>[3x]MNQNLLVTKRDGSTERINLDKIHRVLDWAAEGLHNVSISQVELRSHIQFYDGIKTSDIHETIIKAAADLISRDAPDYQYLAARLAIFHLRKKAYGQFEPPALYDHVVKMVEMGKYDNHLLEDYTEEEFKQMDTFIDHDRDMTFSYAAVKQLEGKYLVQNRVTGEIYESAQFLYILVAACLFSNYPRET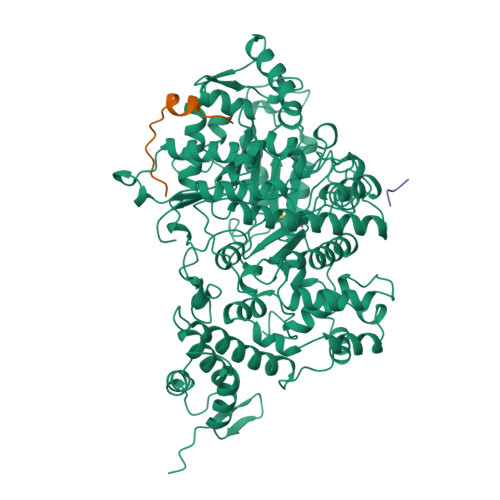RLQYVKRFYDAVSTFKISLPTPIMSGVRTPTRQFSSCVLIECGDSLDSINATSSAIVKYVSQRAGIGINAGRIRALGSPIRGGEAFHTGCIPFYKHFQTAVKSCSQGGVRGGAATLFYPMWHLEVESLLVLKNNRGVEGNRVRHMDYGVQINKLMYTRLLKGEDITLFSPSDVPGLYDAFFADQEEFERLYTKYEKDDSIRKQRVKAVELFSLMMQERASTGRIYIQNVDHCNTHSPFDPAIAPVRQSNLCLDIALPTKPLNDVNDENGEIALCTLSAFNLGAINNLDELEELAILAVRALDALLDYQDYPIPAAKRGAMGRRTLGIGVINFAYYLAKHGKRYSDGSANNLTHKTFEAIQYYLLKASNELAKEQGACPWFNETTYAKGILPIDTYKKDLDTIANEPLHYDWEALRESIKTHGLRNSTLSALMPSETSSQISNATNGIEPPRGYVSIKASKDGILRQVVPDYEHLHDAYELLWEMPGNDGYLQLVGIMQKFIDQSISANTNYDPSRFPSGKVPMQQLLKDLLTAYKFGVKTLYYQNTRDGAEDAQDDLVPSIQDDGCESGACKI;>[4x]YLVGQIDSEVDTDDLSNFQL> GAQVSTQKTGAHETSLSAAGNSIIHYTNINYYKDAASNSANRQDFTQDPSKFTEPV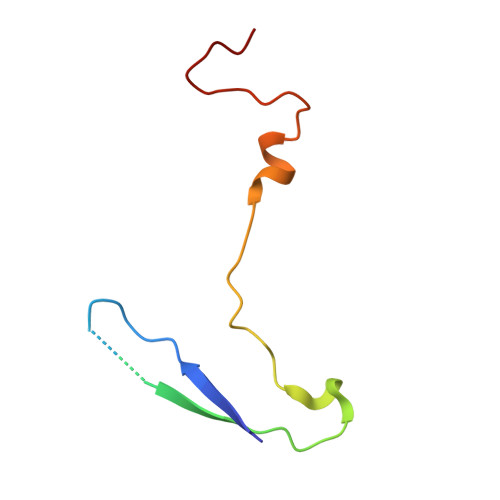KDVMIKSLPAL>MLQFKKTLLSSIAPVLLSIVLANPVIASDAHHAHKGLNYGSFTKEHVLLTPKGYREWVFIGASVTPNELNDDKAAFPEFHNVYIDPTSWGHWKKTGEFRDGTVIVKELAGVGSKASPSGNGYFPGEFNGIEAMVKDSKRYPERPGNWAFFGFESYEAKQGIIQTDETCAACHKEHAAHDMVFTQFYPVLRA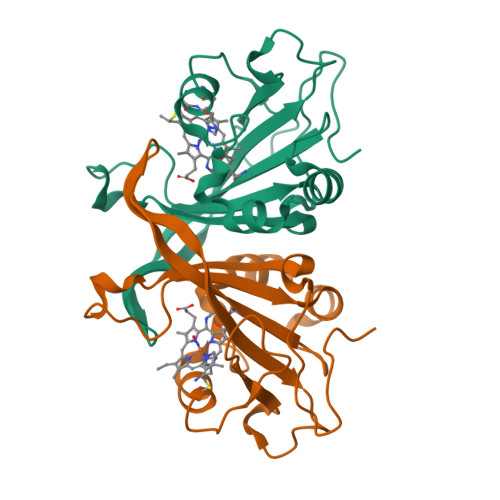GKPSK[4x]Phosphorylation of p6.9 is mediated by protein kinase-1 (PK-1), a protein kinase expressed within the nucleocapsid of lepidopteran-infecting baculoviruses. Here, we present the crystal structure of Cydia pomenella granulovirus PK-1: a serine/threonine protein kinase that, despite being encoded by the baculoviral genome, shares the fold of a eukaryotic protein kinase. Therefore, both the encapsulation and release of the baculoviral genome is regulated by the phosphorylation status of p6.9, thus supporting a pivotal role for post-translational modifications in the baculovirus life cycle. Phylogenetically, PK-1 appears to have originated from its host’s genome, with the greatest similarities to the AGC kinase domain of ribosomal protein S6 kinase A5 (RPS6KA5) homologues in arthropods.

PK-1 exhibited a bi-lobal architecture, comprising a smaller N-terminal lobe (tan) and a large C-terminal lobe (green) that are connected by a short hinge region (purple), which resembles the classical eukaryotic protein kinase fold. The N-lobe contains five β-strands (β1–β5) that form an antiparallel β-sheet, the regulatory αC-helix (dark blue) and an unusual additional α-helix at the very N-terminus that sits atop the N-lobe. The crystal structure contained two PK-1 protomers in the asymmetric unit, which closely associate to form a parallel, side-to-side dimeric assembly. As a consequence of these interactions, the αC helices from each protomer are positioned side-by-side in an antiparallel arrangement and the active sites of each protomer face in opposite directions. Accordingly, co-crystallized AMP was bound in the active site in a conformation analogous to that commonly observed for ATP in eukaryotic protein kinases. Although unusual in protein kinase structures, the entire activation loop was resolved in our PK-1 structure. The activation loop adopted an extended conformation, which appears to have been stabilized by interactions with its dimeric partner, including residues C-terminal to the αE-helix located at the dimeric interface. Our data lead us to propose an unusual mechanism, whereby the dimerization of PK-1 via an atypical dimer interface facilitates constitutive phosphorylation of its substrates. This dimerization mode stabilizes elements typically flexible in kinases, the Gly-rich and activation loops, and by locking the kinase into a rigid, active conformation marked by an intact R-spine and β3-strand K49:αC helix E60 salt bridge, predisposes PK-1 to binding ATP in a productive orientation for catalysis.

>[2x]MNPSKSISRVAQELSKYEILKKLDESDTESYSSVYLCKKKGEHKRFVCKIVKPSTFNSLEFDVHILMRNNPNFIKLHNFVFNDNGESLLIMDYVSDGDLFDFVKMNDTRELRLNEAACKKIIITLVTALNDLHKNNIVHNDVKLENLLYDRKKKRLFVCDYGLSRIVGTPSFYDGTTVYFSPEKIRHEAYQTSFDWWAVGVVAYEILSTEYPFDINEDNEEEMDAIEPKDMLPLYSKPLPTIEHVSKKANDFVRRMLALDINSRLSTYDEIIKHPFLCF>[2x]SRKTYTLTDYLKNTYRLKLYSLRWISDHEYLYKQENNILVFNAEYGNSSVFLENSTFDEFGHSINDYSISPDGQFILLEYNYVKQWRHSYTASYDIYDLNKRQLITEERIPNNTQWVTWSPVGHKLAYVWNNDIYVKIEPNLPSYRITWTGKEDIIYNGITDWVYEEEVFSAYSALWWSPNGTFLAYAQFNDTEVPLIEYSFYSDESLQYPKTVRVPYPKAGAVNPTVKFFVVNTDSLSSVTNATSIQITAPASMLIGDHYLCDVTWATQERISLQWLRRIQNYSVMDICDYDESSGRWNCLVARQHIEMSTTGWVGRFRPSEPHFTLDGNSFYKIISNEEGYRHICYFQIDKKDCTFITKGTWEVIGIEALTSDYLYYISNEYKGMPGGRNLYKIQLSDYTKVTCLSCELNPERCQYYSVSFSKEAKYYQLRCSGPGLPLYTLHSSVNDKGLRVLEDNSALDKMLQNVQMPSKKLDFIILNETKFWYQMILP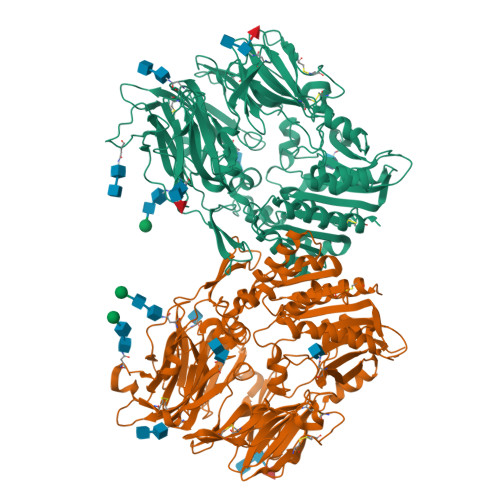PHFDKSKKYPLLLDVFAGPCSQKADTVFRLNWATYLASTENIIVASFDGRGSGYQGDKIMHAINRRLGTFEVEDQIEAARQFSKMGFVDNKRIAIWGWSYGGYVTSMVLGSGSGVFKCGIAVAPVSRWEYYDSVYTERYMGLPTPEDNLDHYRNSTVMSRAENFKQVEYLLIHGTADDNVHFQQSAQISKALVDVGVDFQAMWYTDEDHGIASSTAHQHIYTHMSHFIKQCFSLP>[2x]MNLFQTVFTGSKQALAAAEGIVKQAVDEKGRDYKVAFPDTAYSLPVIFAATGKKITNVGELEGALDIVRSLIVEEEMLDKLLNSGLATAVAAEIIEAAKYVLSDAPYAEPCVGFISDPIIRSLGVPLVTGDIPGVAVILGECPDSETAAKIIKDYQSKGLLTCLVGKVIDQAIEGKVKMGLDLRVIPLGYDVTSVIHVVTIAIRAALIFGGIKGGQLNDILKYTAERVPAFVNAFGPLSELVVSAGAGAIALGFPVLTDQVVPEVPTLLLTQKDYDKMVKTSLEARNIKIKITEIPIPVSFAAAFEGERIRKNDMLAEFGGNKTKAWELVMCADQGEVEDHKIEVIGPDIDTIDKAPGRMPLGMLIKVSGTNMQKDFEPVLERRLHYFLNYIEGVMHVGQRNLTWVRIGKEAFEKGFRLKHFGEVIYAKMLDEFGSVVDKCEVTIITDPGKAEELEGKYAVPRYKERDARLESLVDEKVDTFYSCNLCQSFAPAHVCIVTPERLGLCGAVSWLDAKATLELNPTGPCQAVPKEGVVDENLGIWEKVNETVSKISQGAVTSVTLYSILQDPMTSCGCFECITGIMPEANGVVMVNREFGATTPLGMTFGELASMTGGGVQTPGFMGHGRQFIASKKFMKGEGGLGRIVWMPKELKDFVAEKLNKTAKELYNIDNFADMICDETIATESEEVVKFLEEKGHPALKMDPIM;>MEEKAKSIDQATLQLLDKAKQDGVETVWDRKADMKVQCGFGSAGVCCRNCSMGPCRVSPVPGKGVERGICGATADVIVSRNFARMVAAGTAAHSDHGRSIALSLYHTSKDGDIKVKDENKLKEVAKSFNVETEGRDIYDIAHDVAKEGLSNYGKQLGEVTLPPSLPEKRKELWRK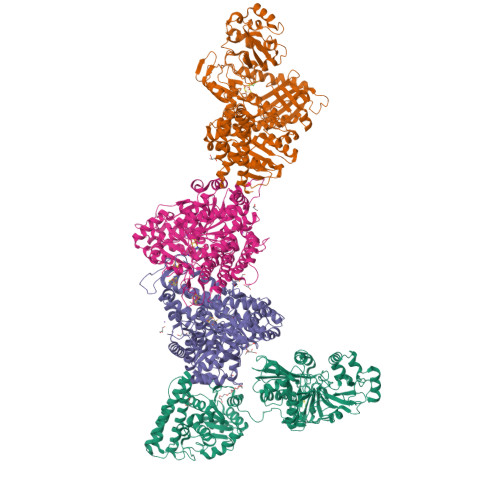LGVYPRAVDREIAAVMHSTHIGCNADAEAMIKMSMRCSLTDGWMGSFMGTEFSDIMFGTPHSIDTEANLGVLEKNSVNVVLHGHEPLLSEMVVEAASDPELVELAKSVGADGINLCGMCCTGNEVSMRHGIKIAGNFMQQELAVVTGAVDGLIVDVQCIMPALAKLSKSYHTKFITTSPKAHITDSIYMEFDEENPLDSAKKILKEAILNFKNRDQSKVMIPELKCKAILGYSVEEIINKLDKVVNTQIGPMQTVKPLADVLVSGVLRGAAAVVGCNNPKVVQDSAHIETIKGLIKNDVIVVVTGCAAQAAAKYGLLQKEAAEKYAGPGLATVCKLVDIPPVLHMGSCVDISRILDLVGRVANLLGVDMSDLPVAGVAPEWMSEKAVAIGTYVVTSGIDTWLGVAPPVTGGPEVVDILTNKMEDWVGAKFFIETDPHKAVEQIVNRMNEKRKKLGI[2x]Lybatides are cysteine-rich and highly constrained peptides. Alignment of lybatides revealed that they contain eight highly conserved cysteine residues arranged in a unique spacing of C-C-C-C-CC-CC, with a sequence identity of 76.5% between the two. Disulfide mapping of lybatides revealed a novel disulfide connectivity of CysI‒CysVI, CysII‒CysVIII, CysIII‒CysVII and CysIV‒CysV. Comparison of its cysteine arrangements, disulfide connectivity and overall three-dimensional structure to other cysteine-rich peptides show that lybatides represent a new family of CRP with an unusual cystine-stabilized helical structure that has not been described in other plant CRPs.

The process was repeated to determine the sequence of the 33-residue Lyba2 as DSCSEYCSNRCPSCDGQTQTQYTLCCINICCPS. There are three copies of the peptide molecule (named A, B and C) per asymmetric unit (ASU) of the crystal. The four disulfide bonds are formed by Cys3‒Cys26, Cys7‒Cys31, Cys11‒Cys30 and Cys14‒Cys25 according to the X-ray structure. Cys3, Cys7 and Cys11 are located in the N terminal loop, which is stabilized via disulfide bonds with Cys26, Cys31 and Cys30 of the π helix. Cys14 is situated at the C-terminus of the one-turn 310 helix and connects with Cys25 of the π helix (molecule A) and α helix (molecules B and C). Instead of the α-helix – α-helix cystine stabilization found in thionins or the α-helix – β-sheets stabilization in plant defensins, the (α + π)-helix in lybatides is stabilized by four disulfide bonds located in two turns (the β-turn 2–6 and the 310-helical turn 12–14) and one loop (7–11) in the N-terminal portion of the peptide. The distortion of the α-helix towards a π-helix in the C-terminal half of lybatides is of interest. This is very likely caused by conformational stress induced by the disulfide bonds at the C-terminus (Cys30 and Cys31). Interestingly, we found that a short polyethylene glycol molecule (PEG, HO-(CH2-CH2-O)3-CH2-CH2-OH, here named “P40”) stabilizes the crystal lattice by filling a cleft between molecule C and its symmetry-related copy C* (symmetry operator: X-1, Y, Z). The majority of its interactions with peptide copies C and C* consist of water-mediated hydrogen bonds.

>DSCSEYCSNRCPSCDGQTQTQYTLCCINICCPS[3x]> GTRKCELQGLWRNELGSNMTISALDVAGTFSGSYQTAV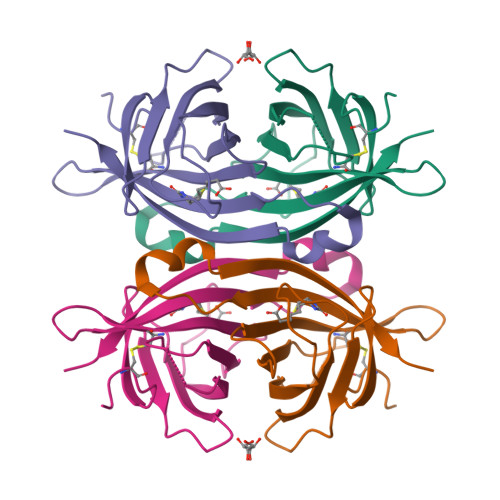TATNKQILVSPLKGAQQPPGTKGQQPTFGFTVQWQFADSTTVFVGQCFVDRRGKEMLEMAWLLREEVPSRKDTWKATRVGTNVFTRVK L-gamma-glutamyl-S-(3-methyl-1,4-dioxo-1,4-dihydronaphthalen-2-yl)-L-cysteinylglycine 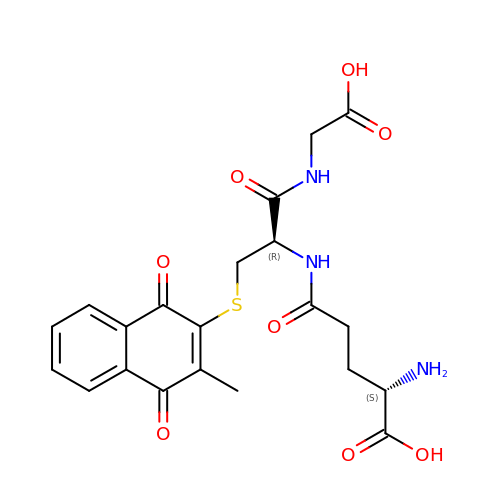| C21 H23 N3 O8 S | BWKXZXMVXPXYDF-KBPBESRZSA-N2-[(2R,5R,6S)-5-hydroxy-1,2,4,5,6,7-hexahydro-3H-2,6-methanoazocino[5,4-b]indol-3-yl]acetamide 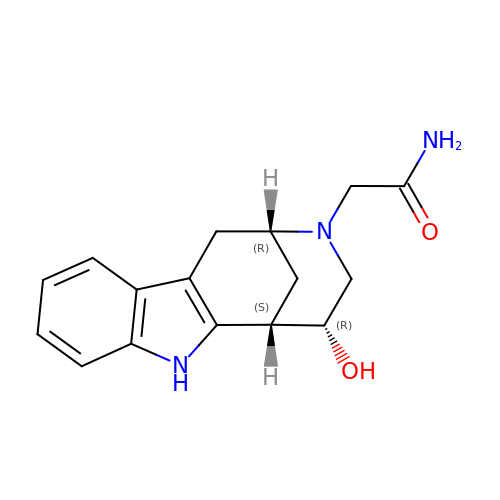| C16 H19 N3 O2 | XUAJXPXSOUOOHU-BHYNMZESSA-N>[2x]MSGKNEADSKDTGWEQIKDKGKIVVATSGTLYPTSYHDTDSGSDK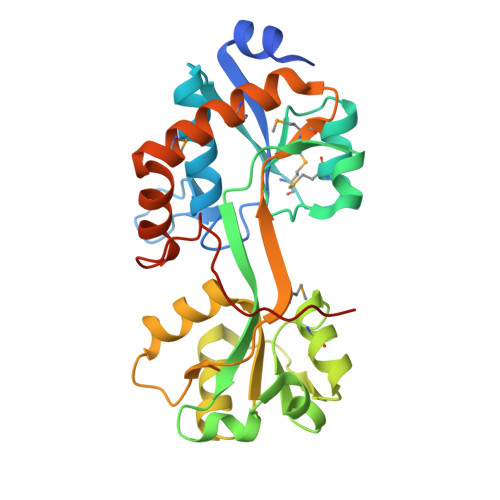LTGYEVEVVREAAKRLGLKVEFKEMGIDGMLTAVNSGQVDAAANDIDVTKDREEKFAFSTPYKYSYGTAIVRKDDLSGIKTLKDLKGKKAAGAATTVYMEVARKYGAKEVIYDNATNEQYLKDVANGRTDVILNDYYLQTLALAAFPDLNITIHPDIKYMPNKQALVMKKSNAALQKKMNEALKEMSKDGSLTKLSKQFFNKADVSKKIDADVQDVDLLEHHHHHH>[2x]MALRFEALYPEGMCPGWSVVVKGKTSSNTSMFEINFLSHPGDQIAFHFNPRFASSRIVCNSFLANHWGKEEVNKTFPFEAKEPFQVEIYSDQDYFHIFIDENKILQYKH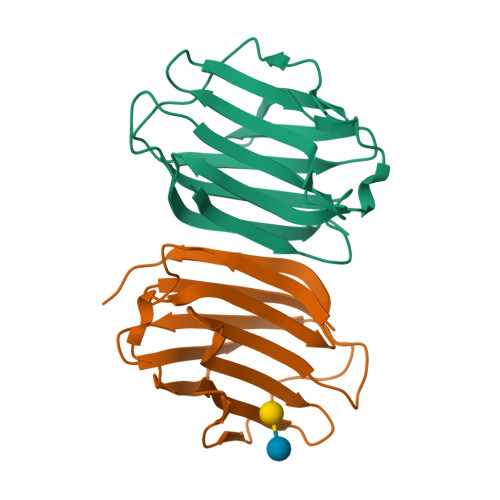RQKQLSSITKLQILNDIEISSVEITKRGLY>SNAMEDLDALWERYREAVRAGGNPQALYQEMVWPALLALWREKPRVYPFPQAFAVSVHTLGTSPEATALAILGAGAERVYVLHTPESARFLPRLRQDTGKDLYPVEIGKSDVEAIYREVKRLLEKHPEVPVALDLTSGTKAMSAGLAAAGFFFQRFYPKVRVVYVDNEDYDPELRRPRAGTEKLRILPNPHEALAEVDALFAKELYGKGEFGQAAAYFRGMVGRTGNQAYALYALLAEMYRAWRALDFGEALKAGRKLLGQLSQNVWLNHPLNARREALEAQVALLEAVDRFLKARDFALKEGVYGLARTLLHLAQEAKEEAAVLAALYAYRALELLLQERLALLGRRAEAPGLSPEEAEALRKALAELLGVLPEEVRLPAKLGLLDLLAFLRLKGDEALGRLSLAELRGLAGALKGRNSALLVHGFDVPSPKAVEGIARLAQGLLQDLEARTALGPLSPEPVPLGF[2x]

In type III-A CRISPR–Cas systems, the RNA-guided multisubunit Csm effector complex targets both single-stranded RNAs and double-stranded DNAs. In addition to the Csm complex, efficient anti-plasmid immunity mediated by type III-A systems also requires the CRISPR-associated protein Csm6. We report the crystal structure of T. thermophilus Csm6 (TtCsm6) at 2.3 Å resolution and show that the protein is a ssRNA-specific endoribonuclease. Csx1 has been shown to be required for the interference activity of a type III-B CRISPR–Cas system in Sulfolobus islandicus. Both Csm6 and Csx1 proteins share an overall architecture defined by an N-terminal CARF domain (CRISPR-associated Rossman fold) and a C-terminal HEPN domain (higher eukaryotes and prokaryotes nucleotide-binding domain) that contains a conserved R-X4-6-H motif.

TtCsm6 crystallization was dependent on the presence of Ni2+ ions, which allowed us to solve the structure using single-wavelength anomalous diffraction (SAD) phasing. The protein crystallized as a homodimer, consistent with size-exclusion chromatography data indicating that the protein is dimeric in solution. The TtCsm6 homodimer resembles an elongated X-shape with overall dimensions of ∼120 Å × 70 Å × 60 Å. Dimerization of TtCsm6 buries ∼2800 Å2 of solvent-accessible surface area per chain and is mediated by two dimer interfaces, one involving the N-terminal CARF domains and the other comprising both the 6H and HEPN domains. In the TtCsm6 structure, the floor of the HEPN domain cleft is lined with side chains of the invariant residues Arg415, Asn416, and His422 from the R-X4-6-H motif. The Asn416/His422 side chain pairs from the two HEPN domains bind a single Ni2+ ion in a tetragonal planar coordination. As TtCsm6 and other HEPN domain ribonucleases are divalent metal-independent enzymes (Anantharaman et al. 2013), the observed Ni2+ ion binding in the putative active site of TtCsm6 might be an artefact due to crystallization in the presence of nickel(II) chloride. In SmCsm6, the R-X4-6-H motif residues reside in an α helix, whereas the TtCsm6 R-X4-6-H motif adopts an irregular loop conformation, suggesting that the TtCsm6 active center might be distorted as a result of Ni2+ binding. Consistent with the observed ssRNA-selective ribonuclease activity of TtCsm6, the width of the cleft would permit binding of a single-stranded nucleic acid substrate, while sterically excluding double-stranded nucleic acids. Taken together, the structural features of TtCsm6 dimer thus suggest that the protein contains two ligand-binding sites: a putative allosteric ligand-binding site at the interface of the CARF domains, and an ssRNA-binding cleft located at the HEPN domain interface, which harbors the ribonuclease active center.>GKISTDKYIFLTPRAYIIVHLLKVGKAKASEISENTQIPYQTVIQNIRWLLAEGYVVKEQKGEEIYYK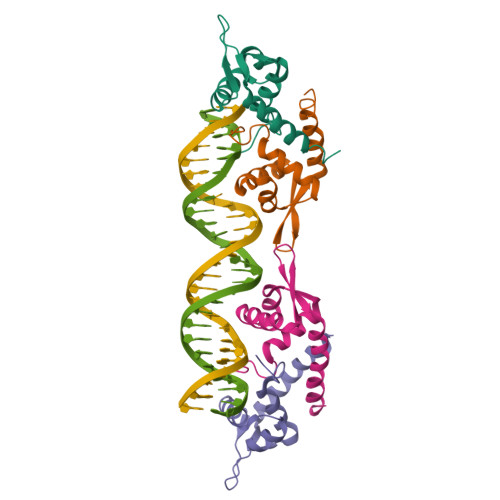LTDKGKQLATAELEKIRKLVEVVQHHHHHH[4x]> L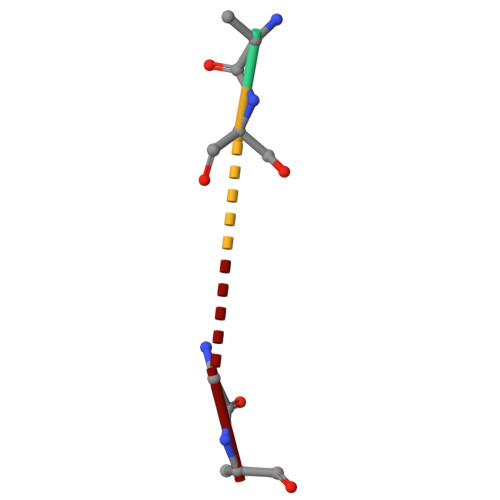SGV>[2x]MGPKSAPLKEIPDVLVDPRTMKRYMRGRFLGKGGFAKCYEITDMDTKEVFAGKVVPKSMLLKPHQKEKMSTEIAIHKSLDNPHVVGFHGFFEDDDFVYVVLEICRRRSLLELHKRRKAVTEPEARYFMRQTIQGVQYLHNNRVIHRNLKLGNLFLNDDMDVKIGDFGLATKIEFDGFRKKTLCGTPNYIAPEVLCKKGHSFEVDIWSLGCILYTLLVGKPPFETSCLKETYIRIKKNEYSV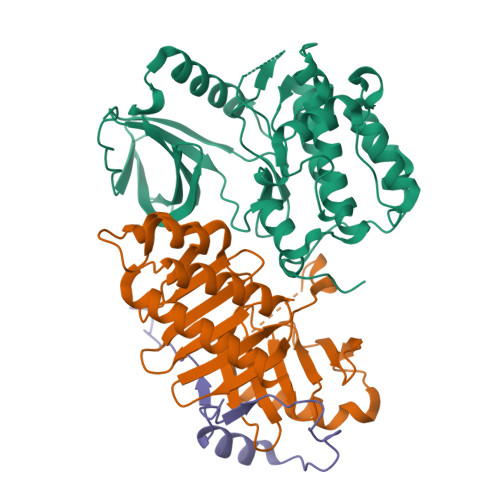PRHINPVASALIRRMLHADPTLRPSVAELLTDEFFTSGYAPMRLPTSCLTVPPRFS;>MQPDTHLTDMLQQLAVVNAAKPSDRGFIRQEEAEDPACIPVFWISKWVDYSDKYGLGYQLSDNSVGVLFNDSTRLIMCADGDSLQYIDRNSLESYLSVRSYPSALSKKITLLKYFRNYMSEHLLKAGANITPREGDELTRLPYLRHWFRTKSAIVLHLSNGTVQINFFQDHTKLILCPLMGAVTYINEKREFYTYKMTLIEEFGCCKELASRLRYARNMVEKLMACKSSTTAATSAR[2x];>MGHHHHHHLDDLVAESPRKEFARINMDGIAVPDEREFDIEADMRPHELEQESDTFGAG[2x]> MASWSHPQFEKMGMLEARELLCERDERTLFSGLSFTLNAGEWVQITGSNGAGKTTLLRLLTGLSRPDAGEVLWQGQPLHQVRDSYHQNLLWIGHQPGIKTRLTALENLHFYHRDGDTAQCLEALAQAGLAGFEDIPVNQLSAGQQRRVALARLWLTRATLWILDQPFTAIDVNGVDRL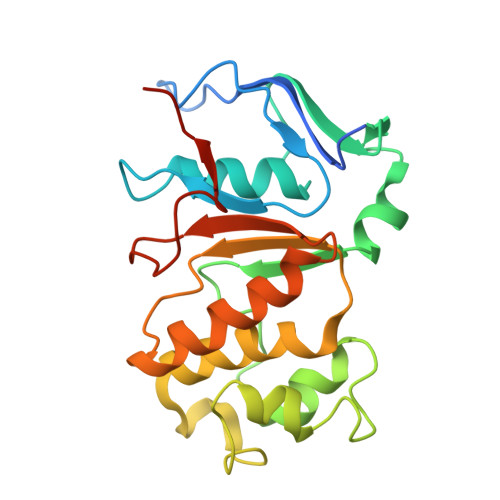TQRMAQHTEQGGIVILTTHQPLNVAESKIRRISLTQTRAA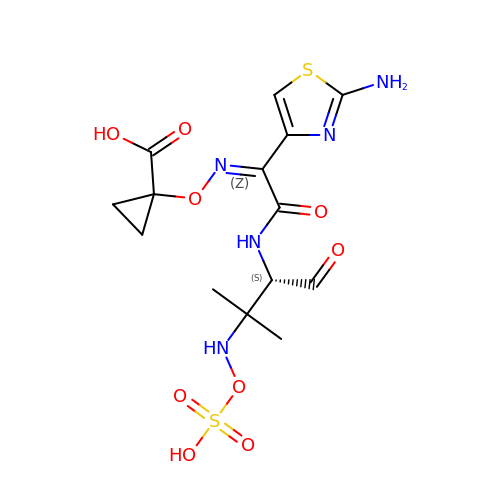1-[(~{Z})-[1-(2-azanyl-1,3-thiazol-4-yl)-2-[[(2~{S})-3-methyl-1-oxidanylidene-3-(sulfooxyamino)butan-2-yl]amino]-2-oxidanylidene-ethylidene]amino]oxycyclopropane-1-carboxylic acid | C14 H19 N5 O9 S2 | IGCRMLSJLQPZRL-ZWJKEBRUSA-N>[2x]SKPKQPPDASPANLLTSLVRAHLDSGPSTAKLDYSKFQELVLPHFGKEDAGDVQQFYDLLSGSLEVIRKWAEKIPGFAELSPADQDLLLEWAFLELFILRLAYRSKPGEGKLIFCSGLVLHRLQCARGFGDWIDSILAFSRSLHSLLVDVPAFACLSALVLITDRHGLQEPRRVEELQNRIASCLKEHVAAVAGEPQPASC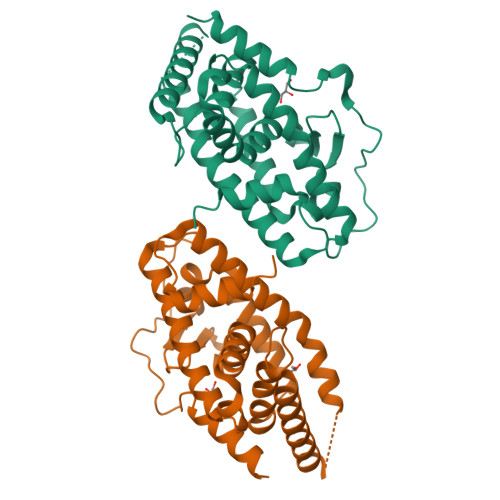LSRLLGKLPELRTLCTQGLQRIFYLKLEDLVPPPPIIDKIFMDTLPFLEHHHHHH> ALPPVAKAAQVVNQTLQLDDSYPDLDSYCRPGASSDYEMQSSDSSWAPFHVVRHHNIPDKVFEHLNAGEVFTKLGLFAEIGYAWASIDSSLFLWDYTHPNPELIGYEEATHTITAVALVPPKPGVFVKTITHVLVVATTSEIILLGVSATPTPSGSKSLTLYSTRMSVHRGGSDVSFIVGTKDGRIFLGGESDTDIHEIFYQQEERWFSSRCGKINHSHPFGSRQQEWLRGLYVDDTRNLLYSLSNRSTIRTYHMEGPEKLTKVIEKDKTSCLRDFAHMADSSPLFTDKTNIVALSPIPATEASKLHLMALTDTGCRLFLSATSSASYTMGGATALAPQSMQLQFVKFPPRESPTRIRTLNGQIIDSQLDKTSRALDPSALGFRFSPGYFFDVVR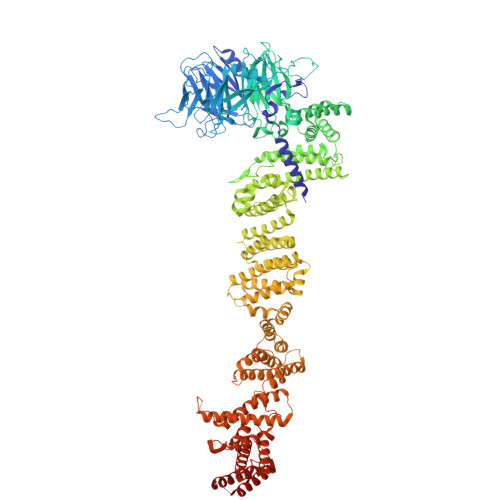KHPNQDMLFVSAPDTGRIKVTQPASALKYFEQGTWIELENGNRTIEIGLTTAPFAAAKQPLGFGNELAVQFDQVPGEFAVLTNTGVHIVRRRRLVDIFAKALGNCVSASDDALEREVRKFINQYGRVETIAAALAVACGQGSDLRTGTGRGMDRNTENLARAAFIEYGGQPRLAESDGKQSVSESVRLSSRHDALALYLTRLVRTLWKAKVVQVGSGSDISSTIPTSKLVTIQENVERLRNFLEANKSTIQGLAPPSERLFGRQEDIANQKEHQALHALQKLMESISEGISFVLMLFDERVSDIYARLDAVSQQQLKDLTYEQLFSQTPGKELAKVLVKAIVNRNIASGANVETVADALRRRCGSFCSPDDVVTFKAQEQLQRASEQAHNSPVLRALLAESLRLFEQVAGSLTPANLTTAVEQYISLKYYAGAIQLCLTVAQQKDRGNTALSWVNDGKPANDSRKKAFDERKICYNLIHQVLDKLESDFAGEPELVDGRPTLAATKRMEAYNVVNDSSDEVFHFDLYEWYIEKGWTDRILSIDSPHVITYLQRLAETDFRHAELLCRFYTTRSRFFEAAQVQTNLAKSDLNISLKDRIILLSRAKGNASVNTIGISRQQQQQLNHEASELLEIAHIQDDLLERLVADPRIPEERKAEIEEFLDGPIRTLTDLFNDYADQANYYDLCLLIFHAADFHNPRTILDTWNNLINQSHFEAEQRREYWEIVQAGGDLPAGVIAPIAEPPLPYVYVSQQIQLIAHRTSLDSLIFPVNSLLPVVCAYAINNGQDASIGADPCWPIQLFLNLGVPHALVVQVLENVLDTQEAPFTGRRRKLVVQWIAMAVDMWVREVERRGAMAAAAASGASGSEAVMGSWVSELLGRADQVLTQIAGTGATLRGGAASDAEEIASLRRTVKGLKRSVD> RYESQLQMVQVTGSSDNEYFYVDFREYEYDLK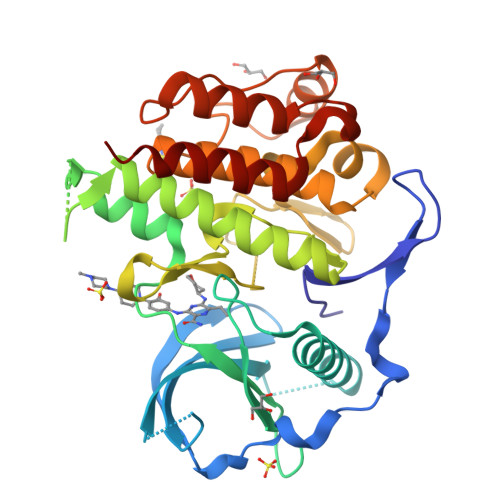WEFPRENLEFGKVLGSGAFGKVMNATAYGISKTGVSIQVAVKMLKEKADSSEREALMSELKMMTQLGSHENIVNLLGACTLSGPIYLIFEYCCYGDLLNYLRSKREKFSEDEIEYENQKRLEEEEDLNVLTFEDLLCFAYQVAKGMEFLEFKSCVHRDLAARNVLVTHGKVVKICDFGLARDIMSDSNYVVRGNARLPVKWMAPESLFEGIYTIKSDVWSYGILLWEIFSLGVNPYPGIPVDANFYKLIQNGFKMDQPFYATEEIYIIMQSCWAFDSRKRPSFPNLTSFLGCQLADAE>[2x]SSIFLLSNVSEDAAQLAEELVREISKKEGTEVRFEKDDGFLTIEVKNLSEERLREIAKALQLIVDVANAERVVRERPGSNLAKKALEIILRAAEELAKLDLKASLKAAVRAAEKVVREQPGSNLAKKALEIILRAAEELAKLPDPEALKEAVKAAEKVVREQPGSELAKKALEIIERAAEELKKSPDPEAQKEAKKAEQKVREERPGS;>[2x]TWQWVLINISEEARQLIEKAVRAISKKEGTEVHFEKDDGVLHIRVKNLHEKRAREIHKVAKLILEVAAAERIVRERPGSNLAKKALEIILRAAEELAKADVDAALEAAVRAAEKVVREQPGSNLAKKALEIILRAAEELAKLPDPEALKEAVKAAEKVVREQPGSELAKKALEIIERAAEELKKSPDPEAQKEAKKAEQKVREERPGS

We set out to design sets of interacting protein pairs for constructing reconfigurable assemblies. We instead sought to use implicit negative design by introducing three properties that collectively make self associated states unlikely to have low free energy: First, in contrast to the flexible coiled coils and helical hairpins in previous designs, we aimed for well folded individual protomers stabilized by substantial hydrophobic cores; this property limits the formation of slowly-exchanging homo-oligomers. Second, we constructed interfaces in which each protomer has a mixed alpha-beta topology and contributes one exposed beta strand to the interface, giving rise to a continuous beta sheet across the heterodimer interface. Our implicit negative design principles enable the de novo design of heterodimer pairs for which the individual protomers are stable in solution and readily form their target heterodimeric complexes upon mixing, unlike previously designed assemblies.

We determined the crystal structures of two class one designs, LHD29 (2.2 Å) and LHD29A53/B53 (2.6 Å) in which both protomers are fused to DHR53. As for unfused LHD29, the interface of LHD29A53/B53 resembles the designed model; at the fusion junction and repeat protein regions, deviations are slightly larger. To further disfavor unwanted homodimeric interactions we rigidly fused designed helical repeat proteins (DHRs) to terminal helices. Since these DHRs have different shapes, they also serve to diversify building block shapes for subsequent higher order assembly design. We used architecture-aware rigid helical fusion to generate two bivalent connector proteins from the crystal-verified fusions of LHD29 and LD101 that allow assembly of a perfectly closed C4-symmetric hetero-oligomeric two-component ring.> PISPIETVPVKLKPGMDGPKVKQWPLTEEKIKALVEICTEMEKEGKISKIGPENPYNTPVFAIKKKDSTKWRKLVDFRELNKRTQDFWEVQLGIPHPAGLKKKKSVTVLDVGDAYFSVPLDEDFRKYTAFTIPSINNETPGIRYQYNVLPQGWKGSPAI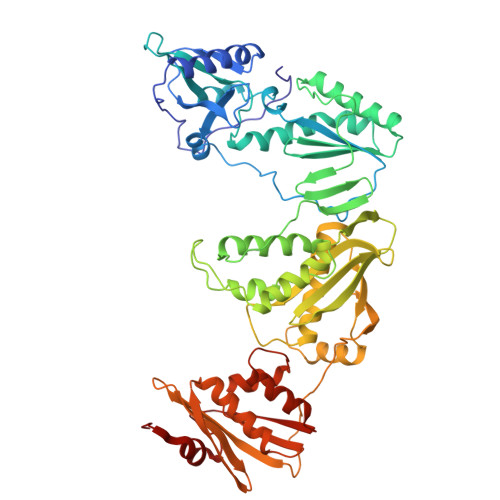FQSSMTKILEPFKKQNPDIVIYQYMDDLLVGSDLEIGQHRTKIEELRQHLLRWGLTTPDKKHQKEPPFLWMGYELHPDKWTVQPIVLPQKDSWTVNDIQKLVGKLNWASQIYPGIKVRQLSKLLRGTKALTEVIPLTEEAELELAENREILKEPVHGVYYDPSKDLIAEIQKQGQGQWTYQIYQEPFKNLKTGKYARMRGAHTNDVKQLTEAVQKITTESIVIWGKTPKFKLPIQKETWETWWTEYWQATWIPEWEFVNTPPLVKLWYQLEKEPIVGAETFYVDGAANRETKLGKAGYVTNKGRQKVVPLTNTTNQKTELQAIYLALQDSGLEVNIVTDSQYALGIIQAQPDKSESELVNQIIEQLIKKEKVYLAWVPAHKGIGGNQQVDKLVSAGIRK>[2x]MSSPEPPTEPPEPDNPTWSTQPTYSNLGQIRAHLLPSKACRLRTPGSLSTNPEPLPPPLPKKILTRTQSLPTRRTLHPSSIQVQPPRRPFLGSHSVDKSQAAVGPACLPAELTFGPADAPLGLSLRDLHSPE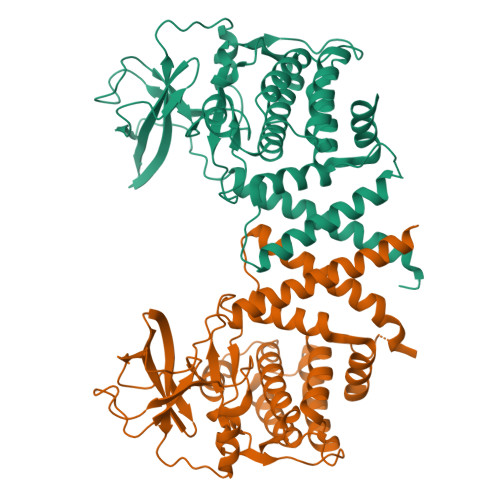AVHTALAARQLQGLRTIYARLRARLMGGHPGPCHPGHSFRLLDSSPCAESGDALYYRVVRAHEDAWHILVAKVPKPGADVPHPWGLELQASLSPHFNLQGLCGLVPEGTLPGAPWRGAVALAAEVPERTVAQWLAEACTQPPEEFVWAVALLLLQLSAALKFLEAWGAALVELRPENLLLVAPRGCATTGPPRLLLTDFGRVCLQPPGPPGSPGPHAPQLGSLLRALLSLAAPSTTPLAAGLELLAAQLTRLRPSASRTRGALQALLWGPGPELRGRGAPLGPWLRALGPWLRVRRGLLVLRLAERAAGGEAPSLEDWLCCEYLAEATESSMGQALALLWDLEGGGGADYKDDDDKGPV>[4x]MPLSQEESTLIERATATINSIPISEDYSVASAALSSDGRIFTGVNVYHFTGGPCAELVVLGTAAAAAAGNLTCIVAIGNENRGILSPCGRCRQVLLDLHPGIKAIVKDSDGQPTAVG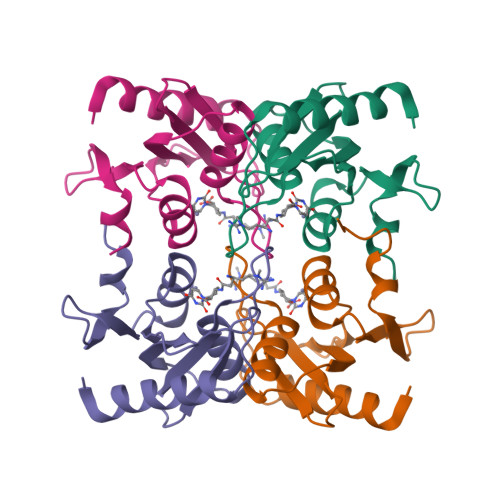IRELLPSGYVWEG> GSSEAKAPTALERVQKEGVLRVITRNSPATYFQDRNGETGFEYELAKRFAERLGVELKIETADNLDDLYAQLSREGGPALAAAGLTPGREDDASVRYSHTYLDVTPQIIYRNGQQRPTRPEDLVGKRIMVLKGSSHAEQLAELKKQYPELKYEESDAVEVVDLLRMVDVGDIDLTLVDSNELAMNQVYFPNVRVAFDFGEARGLAWALPGGDDDSLMNEVNAFLDQAKKEGLLQRLKDRYYGHVDVLGY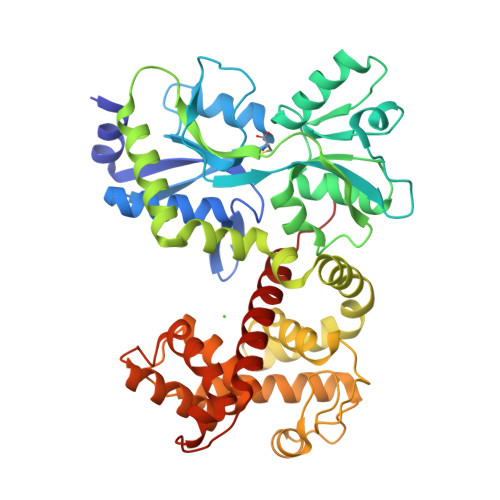VGAYTFAQHLQQRLPRYESHFKQSGKQLDTDWRLLAAIGYQESLWQPGATSKTGVRGLMMLTNRTAQAMGVSNRLDPKQSIQGGSKYFVQIRSELPESIKEPDRSWFALAAYNIGGAHLEDARKMAEKEGLNPNKWLDVKKMLPRLAQKQWYAKTRYGYARGGETVHFVQNVRRYYDILTWVTQPQ> SNAMFAPQGLAQF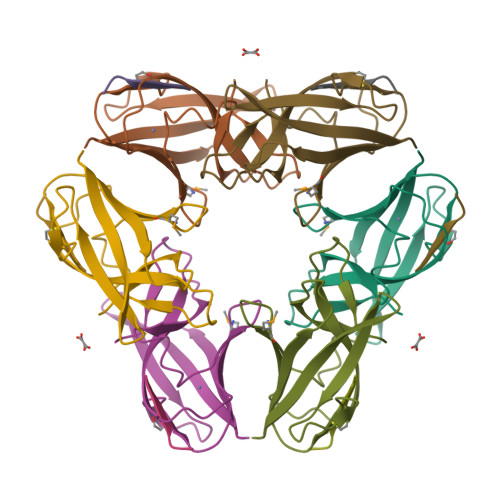IKVNVTLENGEPVFIYTDANGQVCQGDITVTQAGTITYLLNDQTLKGLKFVGVGFVTPFDGIIDAVTISSDGMLVQLVDLDKTPGTTKFQFVLSNTANTLLVLSPD;> PQIINRPQN G protein-coupled receptors (GPCRs) are ubiquitous cellular gatekeepers in eukaryotic organisms. They mediate sensory stimuli and cell signaling, regulating all major physiological processes, and therefore have historically been primary targets in the pharmaceutical industry. Here, we present a simple and efficient method, dubbed Complex-LCP (Crystallization of membrane proteins using transient ligand exchange in LCP), for structure determination of a target GPCR in complex with a panel of different ligands by taking advantage of the SFX method. Concurrent ligand exchange and crystallization is then initiated by overlaying a protein-laden LCP bolus with precipitant solution containing a large excess of the ligand of interest.

To demonstrate the general applicability of the described Complex-LCP method, we applied it to four other GPCRs: serotonin receptors 1B (5-HT1B) and 2B (5-HT2B), adenosine A2A receptor (A2AAR) and melatonin receptor type 1A (MT1). Melatonin receptor MT1 has recently been co-crystallized with several agonists, including two melatonin analogs as well as two drugs: the sleeping aid ramelteon and the atypical antidepressant agomelatine. Since addition of the ligand to the precipitant solution was essential for crystallization in all cases, indicating that ligand-exchange events happen on a timescale comparable to crystallization, we expected MT1 to be a suitable target for our Complex-LCP method. We used the antidepressant agomelatine (Ago) as a transient ligand during crystallization setups and successfully exchanged it for the larger 2-phenylmelatonin (2-PMT), as unambiguously identified in the resulting electron densities.

> GTSQPVLRGDGARPSWLASALACVLIFTIVVDILGNLLVILSVYRNKKLRNAGNIFVVSLAVANLVVAIYPYPLVLMSIFNNGWNFGYLHCQVSAFLMGLSVIGSIWNITGIAIDRYLYICHSLKYDKLYSSKNSLCYVLLIWLLTLAAVLPNLRAGTLQYDPRIYSCTFAQSVSSAYTIAVVVFHFLVPMIIVIFCYLRIWILVLQVRGIDCSFWNESYLTGSRDERKKSLLSKFGMDEGVTFMFIGRFDRGQKGVDVLLKAIEILSSKKEFQEMRFIIIGKGDPELEGWARSLEEKHGNVKVITEMLSREFVRELYGSVDFVIIPSYFEPFGLVALEAMCLGAIPIASAVGGLRDIITNETGILVKAGDPGELANAILKALELSRSDLSKFRENCKKRAMSFSKLKPQDFRNFVTMFVVFVLFAICFAPLNFIGLAVASDPASMVPRIPEWLFVASYYMAYFNSCLNPIIYGLLDQNFRKEYRRIIVSLCTARVFFVDSSN ethyl 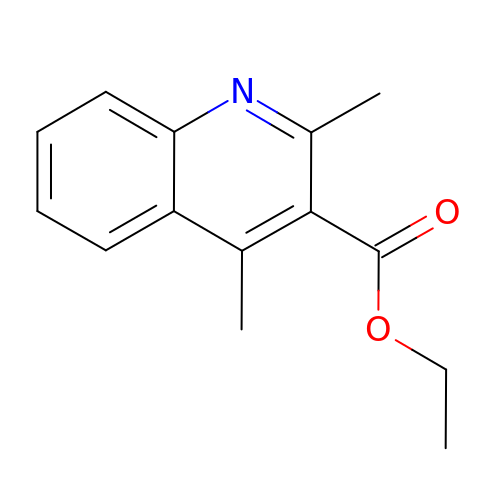2,4-dimethylquinoline-3-carboxylate | C14 H15 N O2 | ASEYONPNBCGPAZ-UHFFFAOYSA-N>GPLGSSAPSVKGVSFDQANNLLIEPARIEEEELTLTILRQTGGLGISIAGGKGSTPYKGDDEGIFISRVSEEGPAARAGVRVGDKLLEVNGVALQGAEHHEAVEALRGAGTAVQMRVWRERM[2x];>EMYYSTAV[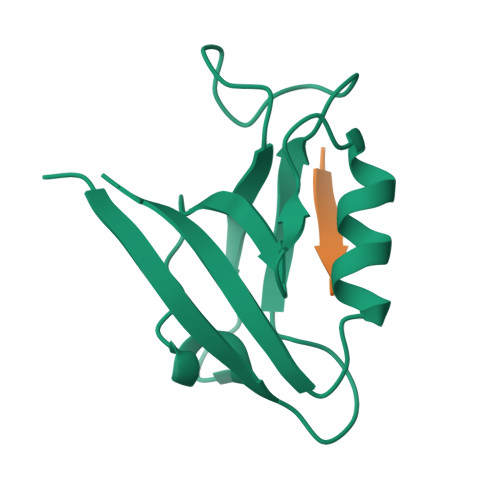2x]>QQDPDPSQLHRSSLVKNLQNIYFLYEGDPVTHENVKSVDQLLSHDLIYNVSGPNYDKLKTELKNQEMATLFKDKNVDIYGVEYYHLCYLCENAERSACIYGGVTNHEGNHLEIPKKIVVKVSIDGIQSLSFDIETNKKMVTAQELDYKVRKYTIDNKQLYTNGPSKYETGYIKFIPKNKESFWFDFFPEPEFTQSKYLMIYKDNE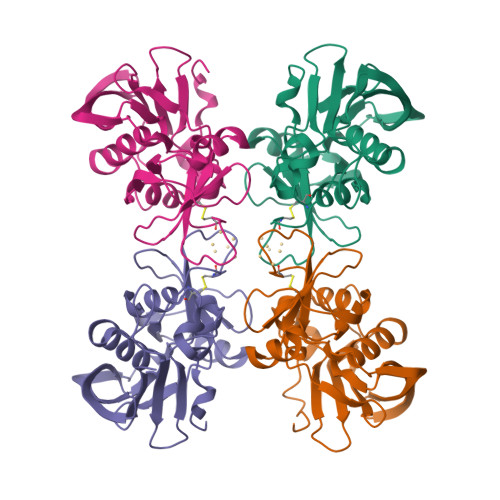TLDNKTSQIEVYLTTK[4x]>[4x]RQVIVPVCMPKIHYSPLKTGLCYDVRMRYHAKIFTSYFEYIDPHPEDPRRIYRIYKILAENGLINDPTLSGVDDLGDLMLKIPVRAATSEEILEVHTKEHLEFIESTEKMSREELLKETEKGDSVYFNNDSYASARLPCGGAIEACKAVVEGRVKNSLAVVRPPGHHAEPQAAGGFCLFSNVAVAAKNILKNYPESVRRIMILDWDIHHGNGTQKSFYQDDQVLYVSLHRF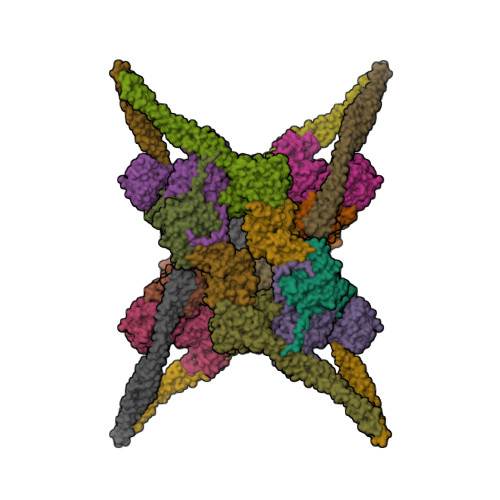EMGKYYPGTIQGQYDQTGEGKGEGFNCNITWPVGGVGDAEYMWAFEQVVMPMGREFKPDLVIISSGFDAADGDTIGQCHVTPSCYGHMTHMLKSLARGNLCVVLEGGYNLDAIARSALSVAKVLIGEPPDELPDPLSDPKPEVIEMIDKVIRLQSKYWNCFRRRHANSGCNFNEPLNDSIISKNFPLQKAIRQQQQHYLSDEFNFVTLPLVSMDLPDNTVLCTPNISESNTIIIVVHDTSDIWAKRNVISGTIDLSSSVIIDNSLDFIKWGLDRKYGIIDVNIPLTLFEPDNYSGMITSQEVLIYLWDNYIKYFPSVAKIAFIGIGDSYSGIVHLLGHRDTRAVTKTVINFLGDKQLKPLVPLVDETLSEWYFKNSLIFSNNSHQCWKENESRKPRKKFGRVLRCDTDGLNNIIEERFEEATDFILDSFE;>[4x]ENSLSTTSKSKRQVIVPVCMPKIHYSPLKTGLCYDVRMRYHAKIFTSYFEYIDPHPEDPRRIYRIYKILAENGLINDPTLSGVDDLGDLMLKIPVRAATSEEILEVHTKEHLEFIESTEKMSREELLKETEKGDSVYFNNDSYASARLPCGGAIEACKAVVEGRVKNSLAVVRPPGHHAEPQAAGGFCLFSNVAVAAKNILKNYPESVRRIMILDWDIHHGNGTQKSFYQDDQVLYVSLHRFEMGKYYPGTIQGQYDQTGEGKGEGFNCNITWPVGGVGDAEYMWAFEQVVMPMGREFKPDLVIISSGFDAADGDTIGQCHVTPSCYGHMTHMLKSLARGNLCVVLEGGYNLDAIARSALSVAKVLIGEPPDELPDPLSDPKPEVIEMIDKVIRLQSKYWNCFRRRHANSGCNFNEPINDSIISKNFPLQKAIRQQQQHYLSDEFNFVTLPLVSMDLPDNTVLCTPNISESNTIIIVVHDTSDIWAKRNVISGTIDLSSSVIIDNSLDFIKWGLDRKYGIIDVNIPLTLFEPDNYSGMITSQEVLIYLWDNYIKYFPSVAKIAFIGIGDSYSGIVHLLGHRDTRAVTKTVINFLGDKQLKPLVPLVDETLSEWYFKNSLIFSNNSHQCWKENESRKPRKKFGRVLRCDTDGLNNIIEERFEEATDFILDSFE;>KVYYLPVTLTQFQKDLSEILISLHAKSFKASIIGEPQADAVNKPSGLPAGPETHPYPTLSQRQLTYIFDSNIRAIANHPSLLVDHYMPRQLLRMEPTESSIAGSHKFQVLNQLINSICFRDREGSPNEVIKCAIIAHSIKELDLLEGLILGKKFRTKRLSGTSLYNEKHKFPNLPTVDSTINKDGTPNSVSSTSSNSNSTSYTGYSKDDYDYSVKRNLKKRKINTDDWLFLATTKHLKHDQYLLANYDIDMIISFDPMLEVELPALQVLRNNANKDIPIIKLLVQNSPDHYLLDSEIKNSSVKSSHLSNNGHVDDSQEYEEIKSSLLYFLQARNAPVNNCEIDYIKLVKCCLEGKDCNNILPVLDLITLDEASKDSSDSGFWQPQLTKLQYSSTELPLWDGPLDIKTYQTELMHRAVIRLRDIQDEYAKGTVPLYEKRLNETQRQNQLDEIKNSVGLTFKKKQEVEKSINDSEKRLKHAMTESTKLQNKINHLLKNRQELENFNKLPSNTISSENHLEEGSALADKLKEYIDKNATLFNKLKELQQANAEKSKLNDELRSKYQIESSKAAESAQTLKILQESMKSLENEVNGPLTKFSTESLKKELERLQNDFQSLKARNKFLKNYITL[4x];>SGDYWLPTTMSLYQKELTDQIVSLHYSDILRYFETSHYKEDVILESMKTMCLNGSLVATHPYLLIDHYMPKSLITRDVPAHLAENSGKFSVLRDLINLVQEYETETAIVCRPGRTMDLLEALLLGNKVHIKRYDGHSIKSKQKANDFSCTVHLFSSEGINFTKYPIKSKARFDMLICLDTTVDTSQKDIQYLLQYKRERKGLERYAPIVRLVAINSIDHCRLFFGKKFDKNSREYLENVTAAMVILRDRLGTLPPDLRPIYSQKLHYLVEWLENPTVPWPLPDIYPLKQYTSMDVERSLLTEVHFKNSSNVNYHLSSGIITHKLIQSMGEVYMDICVQKQELDDYSCLDDLQNDHLKFFSNEDEKIIKEYETVLRTNNENLNRSHELEVENNLKFSQIETLEKDIETLKGSLMAQGETLSKLKDAFVKTDNVQDEIEKEERVSVSRDTEKKYMEQEIKRAVDAIRENEEETHKLNEKQNGLESELKLKFEKSEISTKELNEKIGFLKKELKLENDLNEELVGQLSKTMDNLENLTIPRVRTQ[4x]>ATFDILNKCTYTVWAAASPGGGRRLDSGQSWTITVNPGTTNARIWGRTSCTFDANGRGKCETGDCNGLLECQGYGSPPNTLAEFALNQPNNLDYIDISLVDGFNIPMDFSGCRGIQCSVDINGQCPSELKAPGGCNNPCTVFKTNEYCCTDGPGSCGPTTYSKF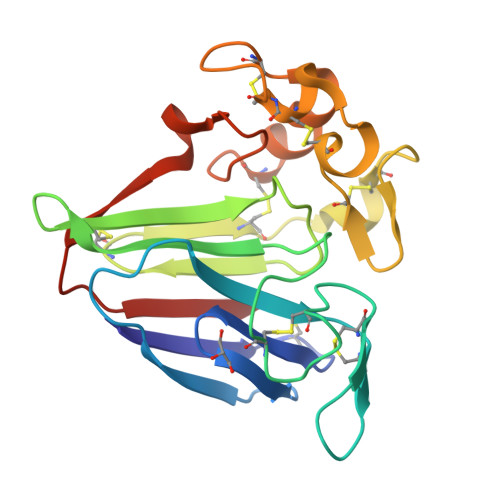FKDRCPDAYSYPQDDKTSLFTCPSGTNYKVTFCP[2x]{[(4-benzylphenyl)amino]methylene}bis(phosphonic acid) | 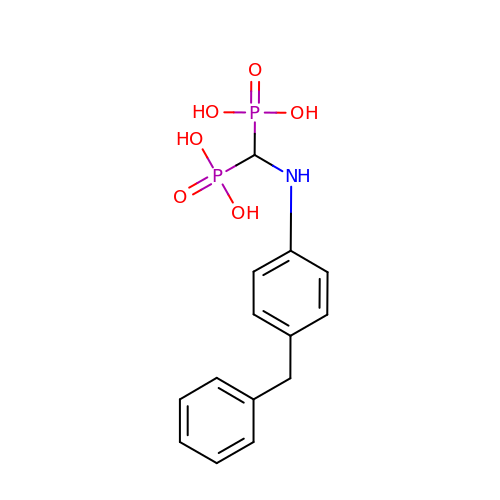C14 H17 N O6 P2 | UUWAWXLKQDUPIO-UHFFFAOYSA-N> SGAFEDRDPTQFEERHLKFLQQLGKGNFGSVEMCRYDPLQDNTGEVVAVKKLQHSTEEHLRDFEREIEILKSLQHDNIVKYKGVCYSAGRRNLKLIMEYLPYGSLRDYLQKHKERIDHIKLLQYTSQICKGMEYLGTKRYIHRDLATRNILVENENRVKIGDFGLTKVLPQDKEYYKVKEPGESPIFWYAPESLTESKFSVASDVWSFGVVLYELFTYIEKSKSPPAEFMRMIGNDKQGQMIVFHLIELLKNNGRLPRPDGCPDEIY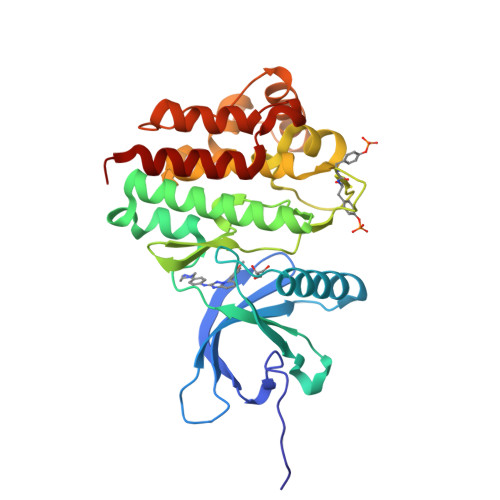MIMTECWNNNVNQRPSFRDLALRVDQIRDNMAG> SAASGRAGRGTLDPRLAQIYSGERRMGDRNTAL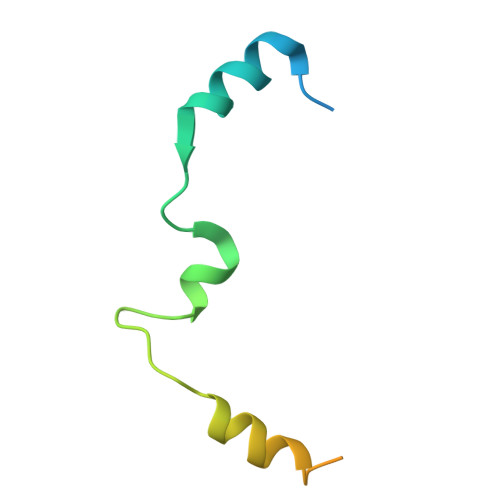RGIKPTDFSHVRKLAAPFVTRKPGAAPSAGVGASATLALNQ> MVSMKDFSGAELYTLEEYQYGKFEARMKMAAASGTVSSMFLYQNGSEIADGRPWVEVDIEVLGKSPGSFQSNIITGKAGAQKTSEKHHAVSPAADQAFHTYGLEWTPNYVRWTVDGQEVRKTEGGQVSNLTGTQGLRFNLWSSESAAWVGQFDESKLPLFQFINWVKVYKYTPGQGEGGSDFTLDWTDNFDTFDGSRWGKGDYTFDGNRVDLTDKN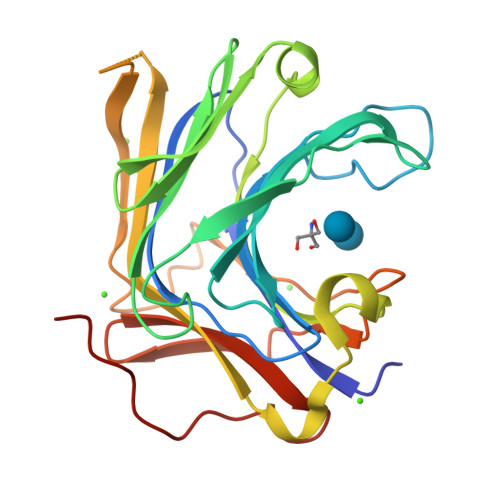IYSRDGMLILALTRKGQESFNGQVPRDDEPAPL>MAYWLMKSEPDELSIEALARLGEARWDGVRNYQARNFLRAMSVGDEFFFYHSSCPQPGIAGIARITRAAYPDPTALDPESHYHDAKATTDKNPWSAVDVAHVQTFPRVLELGRLKQQAGLVELPLV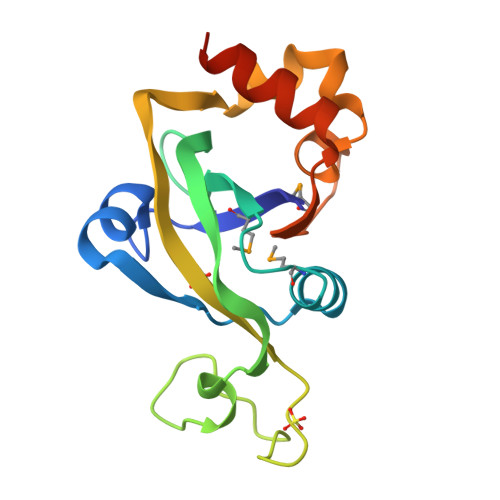QKGSRLSVMPVTPEQWAVIVALRLEHHHHHH[3x]> ETF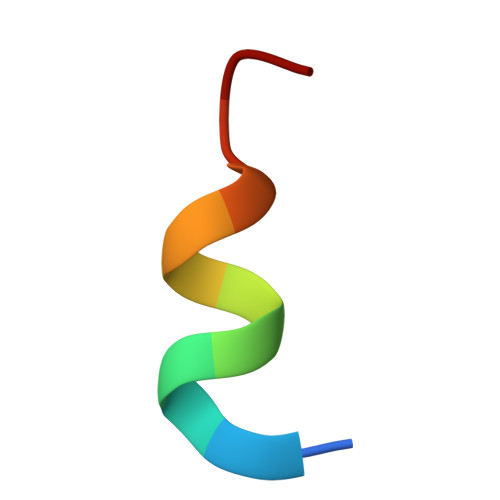EHWWSQLLS The Rpd3 small (Rpd3S) complex recognizes histone H3 trimethylation on lysine 36 (H3K36me3) and deacetylates histones H3 and H4 at multiple sites across transcribed regions. The Rpd3S histone deacetylase (HDAC) complex recognizes H3K36me3 at coding regions and suppresses transcription from cryptic promoters via its deacetylase activity in yeast. Here we solved the cryo-electron microscopy structures of Saccharomyces cerevisiae Rpd3S in its free and H3K36me3 nucleosome-bound states. We demonstrated a unique architecture of Rpd3S, in which two copies of Eaf3–Rco1 heterodimers are asymmetrically assembled with Rpd3 and Sin3 to form a catalytic core complex.

For structural analysis, we co-expressed full-length S. cerevisiae Rpd3, Sin3, Rco1, Eaf3 and Ume1 in a baculovirus–insect cell system and successfully reconstituted the Rpd3S holo-enzyme. Next, we performed single-particle cryo-EM analysis and acquired an overall structural map of Rpd3S at 3.2 Å resolution. Using a focused refinement strategy, we obtained 2.7 Å and 3.2 Å maps of two local regions, the head–bridge–right arm and the left arm of the Rpd3S complex, which enabled de novo model building of approximately 1,800 residues of Rpd3S components with high accuracy. In the structural model, we identified one copy of Rpd3 and Sin3, and two copies of Eaf3 and Rco1. The modelled structure contains residues 664–1322 of Sin3, 17–384 of Rpd3, 220–401 of Eaf3-A, 221–374 of Eaf3-B, 107–565 of Rco1-A and 262–358 of Rco1-B, which constitute a catalytic core complex with Rpd3 positioned at the centre. Although Ume1 exists as a stoichiometric component of Rpd3S, its map is missing. Cross-linking mass spectrometry (XL-MS) further confirmed the existence of Ume1, which mainly interacts with the C-terminal tail of Sin3. Both the Sin3 C-terminal tail and Ume1 are invisible in the map, suggesting their flexible disposition. The two highly integrated MRG–PHD1–MID modules constitute the right and left arms of the Rpd3S complex, which use distinct surfaces for asymmetric Rpd3S assembly. Rpd3 is wrapped around by discrete regions of Sin3, Rco1-A and Eaf3-A, including HID-N, loopS, four-helix-finger (FHF) and HID-C of Sin3 HID domain, PHD1 and PHD2 fingers of Rco1-A, and a C-terminal helix tail (αE) of Eaf3-A from the front surface, as well as an extended α–β-coil (αβC) motif of Rco1-A from the back surface. In the Rpd3S complex, we observed that a long α-helix of Sin3 (α1) within the FHF motif covers the basic surface of Rpd3 and inserts two Glu fingers (Glu811 and Glu812) into the inositol phosphate-binding pocket.

> MSQVWHNSNSQSNDVATSNDATGSNERNEKEPSLQGNKPGFVQQQQRITLPSLSALSTKEEDRRDSNGQQALTSHAAHILGYPPPHSNAMPSIATDSALKQPHEYHPRPKSSSSSPSINASLMNAGPAPLPTVGAASFSLSRFDNPLPIKAPVHTEEPKSYNGLQEEEKATQRPQDCKEVPAGVQPADAPDPSSNHADANDDNNNNENSHDEDADYRPLNVKDALSYLEQVKFQFSSRPDIYNLFLDIMKDFKSQAIDTPGVIERVSTLFRGYPILIQGFNTFLPQGYRIECSSNPDDPIRVTTPMGTTTVNNNISPSGRGTTDAQELGSFPESDGNGVQQPSNVPMVPSSVYQSEQNQDQQQSLPLLATSSGLPSIQQPEMPAHRQIPQSQSLVPQEDAKKNVDVEFSQAISYVNKIKTRFADQPDIYKHFLEILQTYQREQKPINEVYAQVTHLFQNAPDLLEDFKKFLPDSSASANQQVQHAQQHAQQQHEAQMHAQAQAQAQAQAQVEQQKQQQQFLYPASGYYGHPSNRGIPQQNLPPIGSFSPPTNGSTVHEAYQDQQHMQPPHFMPLPSIVQHGPNMVHQGIANENPPLSDLRTSLTEQYAPSSIQHQQQHPQSISPIANTQYGDIPVRPEIDLDPSIVPVVPEPTEPIENNISLNEEVTFFEKAKRYIGNKHLYTEFLKILNLYSQDILDLDDLVEKVDFYLGSNKELFTWFKNFVGYQEKTKCIENIVHEKHRLDLDLCEAFGPSYKRLPKSDTFMPCSGRDDMCWEVLNDEWVGHPVWASEDSGFIAHRKNQYEETLFKIEEERHEYDFYIESNLRTIQCLETIVNKIENMTENEKANFKLPPGLGHTSMTIYKKVIRKVYDKERGFEIIDALHEHPAVTAPVVLKRLKQKDEEWRRAQREWNKVWRELEQKVFFKSLDHLGLTFKQADKKLLTTKQLISEISSIKVDQTNKKIHWLTPKPKSQLDFDFPDKNIFYDILCLADTFITHTTAYSNPDKERLKDLLKYFISLFFSISFEKIEESLYSHKQNVSESSGSDDGSSIASRKRPYQQEMSLLDILHRSRYQKLKRSNDEDGKVPQLSEPPEEEPNTIEEEELIDEEAKNPWLTGNLVEEANSQGIIQNRSIFNLFANTNIYIFFRHWTTIYERLLEIKQMNERVTKEINTRSTVTFAKDLDLLSSQLSEMGLDFVGEDAYKQVLRLSRRLINGDLEHQWFEESLRQAYNNKAFKLYTIDKVTQSLVKHAHTLMTDAKTAEIMALFVKDRNASTTSAKDQIIYRLQVRSHMSNTENMFRIEFDKRTLHVSIQYIALDDLTLKEPKADEDKWKYYVTSYALPHPTEGIPHEKLKIPFLERLIEFGQDIDGTEVDEEFSPEGISVSTLKIKIQPITYQLHIENGSYDVFTRKATNKYPTIANDNTQKGMVSQKKELISKFLDCAVGLRNNLDEAQKLSMQKKWENLKDSIAKTSAGNQGIESETEKGKITKQEQSDNLDSSTASVLPASITTVPQDDNIETTGNTESSDKGAKIQ;> MVYEATPFDPITVKPSDKRRVAYFYDADVGNYAYGAGHPMKPHRIRMAHSLIMNYGLYKKMEIYRAKPATKQEMCQFHTDEYIDFLSRVTPDNLEMFKRESVKFNVGDDCPVFDGLYEYCSISGGGSMEGAARLNRGKCDVAVNYAGGLHHAKKSEASGFCYLNDIVLGIIELLRYHPRVLYIDIDVHHGDGVEEAFYTTDRVMTCSFHKYGEFFPGTGELRDIGVGAGKNYAVNVPLRDGIDDATYRSVFEPVIKKIMEWYQPSAVVLQCGGDSLSGDRLGCFNLSMEGHANCVNYVKSFGIPMMVVGGGGYTMRNVARTWCFETGLLNNVVLDKDLPYNEYYEYYGPDYKLSVRPSNMFNVNTPEYLDKVMTNIFANLENTKYAPSVQLNHTPRDAEDLGDVEEDSAEAKDTKGGSQYARDLHVEHDNEFY;>[2x]MVDLEQEFALGGRCLAFHGPLMYEAKILKIWDPSSKMYTSIPNDKPGGSSQATKEIKPQKLGEDESIPEEIINGKCFFIHYQGWKSSWDEWVGYDRIRAYNEENIAMKKRLANEAKEAKKSLLEQQKKKKLSTSLGGPSNGGKRKGDSRSNASISKSTSQSFLTSSVSGRKSGRSSANSLHPGSSLRSSSDQNGNDDRRRSSSLSPNMLHHIAGYPTPKISLQIPIKLKSVLVDDWEYVTKDKKICRLPADVTVEMVLNKYEHEVSQELESPGSQSQLSEYCAGLKLYFDKCLGNMLLYRLERLQYDELLKKSSKDQKPLVPIRIYGAIHLLRLISVLPELISSTTMDLQSCQLLIKQTEDFLVWLLMHVDEYFNDKDPNRSDDALYVNTSSQYEGVALGM;> MDTSKKDTTRSPSHSNSSSPSSSSLSSSSSKEKKRPKRLSSQNVNYDLKRRKIITSEGIERSFKNEHSNLAVEDNIPEEEPKELLEKDSKGNIIKLNEPSTISEDSKVSVTGLPLNKGPSEKIKRESLWNYRKNLGGQSNNSEMTLVPSKRFTQVPKNFQDLNRNDLKTFLTENMTEESNIRSTIGWNGDIINRTRDREPESDRDNKKLSNIRTKIILSTNATYDSKSKLFGQNSIKSTSNASEKIFRDKNNSTIDFENEDFCSACNQSGSFLCCDTCPKSFHFLCLDPPIDPNNLPKGDWHCNECKFKIFINNSMATLKKIESNFIKQNNNVKIFAKLLFNIDSHNPKQFQLPNYIKETFPAVKTGSRGQYSDENDKIPLTDRQLFNTSYGQSITKLDSYNPDTHIDSNSGKFLICYKCNQTRLGSWSHPENSRLIMTCDYCQTPWHLDCVPRASFKNLGSKWKCPLHSPTKVYKKIHHCQEDNSVNYKVWKKQRLINKKNQLYYEPLQKIGYQNNGNIQIIPTTSHTDYDFNQDFKITQIDENSIKYDFFDKIYKSKMVQKRKLFQFQESLIDKLVSNGSQNGNSEDNMVKDIASLIYFQVSNNDKSSNNKSASKSNNLRKLWDLKELTNVVVPNELDSIQFNDFSSDEIKHLLYLKKIIESKPKEELLKFLNIENPENQSE;> MDTSKKDTTRSPSHSNSSSPSSSSLSSSSSKEKKRPKRLSSQNVNYDLKRRKIITSEGIERSFKNEHSNLAVEDNIPEEEPKELLEKDSKGNIIKLNEPSTISEDSKVSVTGLPLNKGPSEKIKRESLWNYRKNLGGQSNNSEMTLVPSKRFTQVPKNFQDLNRNDLKTFLTENMTEESNIRSTIGWNGDIINRTRDREPESDRDNKKLSNIRTKIILSTNATYDSKSKLFGQNSIKSTSNASEKIFRDKNNSTIDFENEDFCSACNQSGSFLCCDTCPKSFHFLCLDPPIDPNNLPKGDWHCNECKFKIFINNSMATLKKIESNFIKQNNNVKIFAKLLFNIDSHNPKQFQLPNYIKETFPAVKTGSRGQYSDENDKIPLTDRQLFNTSYGQSITKLDSYNPDTHIDSNSGKFLICYKCNQTRLGSWSHPENSRLIMTCDYCQTPWHLDCVPRASFKNLGSKWKCPLHSPTKVYKKIHHCQEDNSVNYKVWKKQRLINKKNQLYYEPLQKIGYQNNGNIQIIPTTSHTDYDFNQDFKITQIDENSIKYDFFDKIYKSKMVQKRKLAQFQESLIDKLVSNGSQNGNSEDNMVKDIASLIYFQVSNNDKSSNNKSASKSNNLRKLWDLKELTNVVVPNELDSIQFNDFSSDEIKHLLYLKKIIESKPKEELLKFLNIENPENQSE The mucolytic human gut microbiota specialist Akkermansia muciniphila is proposed to boost mucin-secretion by the host, thereby being a key player in mucus turnover. Mucin glycan utilization requires the removal of protective caps, notably fucose and sialic acid, but the enzymatic details of this process remain largely unknown. Here, we describe the specificities of ten A. muciniphila glycoside hydrolases, which collectively remove all known sialyl and fucosyl mucin caps including those on double-sulfated epitopes. Structural analyses revealed an unprecedented fucosidase modular arrangement and explained the sialyl T-antigen specificity of a sialidase of a previously unknown family.

Uniquely, AmGH181 displayed exclusive specificity towards the sialyl-T-antigen amongst the tested O-glycans, which was not hindered by α2,6-sialyation or β1,6-substitution of the GalNAc unit. To explain the strict specificity, we determined three structures of AmGH181: in ligand free form, bound with the transition-state inhibitor DANA (N-Acetyl-2,3-dehydro-2-deoxyneuraminic acid), and bound to both the T-antigen disaccharide (GNB) and DANA, which provides a mimic for a transition state-like substrate complex. Comparison of the ligand-free and the ligand-bound structures of AmGH181 revealed the flipping of a tryptophan (W298, 56.3 % conserved within GH181) in the ligand-bound structures. This conformational change positions W298 to stack onto the GalNAc unit of the T-antigen, thereby defining subsite +2. The invariant histidine (H411) from domain B forms potential hydrogen bonds to the Gal and GalNAc units. Thus, W298 and H390 form a “sugar tong” that restricts the T-antigen disaccharide. The galactosyl at subsite +1 stacks onto an invariant tryptophan (W212) and is additionally recognized by two hydrogen bonds. An invariant aspartate (D345), unique for GH181, is hydrogen bonded to the Gal C3-OH group at subsite +1. Collectively, these aromatic stacking and polar interactions provide a plausible explanation for the strict specificity of the enzyme. The first site is adjacent to the active site, where an inhibitor molecule was modelled, whereas a galactose unit was modelled at the second binding site located on the opposite side of the catalytic site.

>[2x]MAPVPEPEVVATPPADAGRGLIRVDSREIRHYSGTRKEPDYLVSRDNGKTWEMKAAPAGYPPNYGGIPKESPAIVRNPLTREFIRVQPIGGFVFLSRGGLDGKWLAVTNDGKLEEDWKDPEKRKNLKKLGGIMRTPVFVNKGRRVIVPFHNMGGGTKFHISDDGGLTWHVSRNGVTSPRHEARPPHQGVRWFNNAVEATVLEMKDGTLWALARTSQDQAWQAFSKDYGETWSKPEPSRFFGTLTMNTLGRLDDGTIVSLWTNTMALPENATAGNGTWEDVFTNRDSHHIAMSGDEGKTWYGFREIILDEHRNHPGYATLDGPEDRGKHQSEMVQLDKNRILISLGQHKNHRRLVIVDRRWVGAKTRATQTGKDLDSQWTIHTYIPQKKGHCSYNRKPSAELVQDPSGGTKKVLQIKRLDDPELVNEKSNVDYRNGGATWNFPNGTTGLVKFRFRVVDGEQADDSGLQVSLTDRLFNACDSTTKDYALFTFPIRLKPAPHLLLGMKKVPFTPGAWHEISLLWQGGQAVVSLDGKKAGTLKMANKSPNGASYIHFISTGSQPDAGILLDTVNARVKLE The Hippo pathway is vital for organ growth control and tissue homeostasis, and its dysregulation has been linked to various human cancers. Upon activation MST1/2 phosphorylates LATS1/2 and MOB1 to support formation of an active MOB1/LATS complex, which phosphorylates YAP/TAZ, promoting its cytoplasmic retention and/or degradation. Thus, the Hippo core pathway can act through distinct kinases, with MOB1 acting as a fundamental signal adaptor that can interact with the Hippo core kinases MST1/2, LATS1/2, and NDR1/216, 19–22. Biochemical evidence suggests that MOB1 can associate with the highly conserved N-terminal regulatory domain (NTR) of NDR/LATS kinases to promote their activities.

To delineate the interaction of MOB1 with NDR2 on the atomic level, we determined the crystal structure of the MOB1/NDR2 complex at 2.1 Å using purified MOB1 (residues 33–216) and the NTR of NDR2 (residues 25–88). The structure of MOB1 adopts a globular shape consisting of nine α-helices (α1–α9) and two β-strands, as reported for unbound human MOB119, 32, frog MOB133, and yeast Mob1p34. The central intermolecular interactions between MOB1 and NDR2 are hydrogen bonds and van der Waals interactions, with the two antiparallel α-helices of NDR2 representing two interaction interfaces. In the α1 helix Lys25, Leu28, Tyr32, Leu35, and Ile36 of NDR2 interact with Leu36, Gly39, Leu41, Ala44, Gln67, Met70, Leu71, Leu173, Gln174, and His185 of MOB1. In the α2 helix Arg42, Leu78, Arg79, and Arg82 of NDR2 interact with Glu51, Glu55, Trp56, Val59, Phe132, Pro133, Lys135, and Val138 of MOB1. MOB1(Q67A) and MOB1(H185A) mutants did not interact with NDR2, illustrating that the observed MOB1/NDR2 interaction is specific. The overall crystal structure of MOB1 bound to NDR2 is very similar to the previously reported structures of MOB1/LATS119, 20. Most significantly, we discovered that His646 of LATS1 bonds with Asp63 of MOB1 supported by a cluster of surrounding residues involving Phe642, Met643, Gln645, Val647, and Val65019, while Phe31 of NDR2 does not interact with Asp63 of MOB1. Consequently, our structural comparison suggests that Asp63 of MOB1 specifically bonds with LATS kinases through His646, which is conserved in human LATS1/2 and fly Wts, but replaced by a bulky Phe/Tyr residue in human NDR1/2 and fly Trc. MOB1/NDR2 complex formation is dramatically increased by prior MST1/2 phosphorylation of MOB1, while the MOB1/LATS1 interaction appears to be fully dependent on MST1/2 phosphorylation of MOB1.

>AAHHSSGHMEATLGSGNLRQAVMLPEGEDLNEWIAVNTVDFFNQINMLYGTITEFCTEASCPVMSAGPRYEYHWADGTNIKKPIKCSAPKYIDYLMTWVQDQLDDETLFPSKIGVPFPKNFMSVAKTILKRLFRVYAHIYHQHFDSVMQLQEEAHLNTSFKHFIFFVQEFNLIDRRELAPLQELIEKLGSKDR[2x];>[2x]SSGHMKLTLENFYSNLILQHEERETRQKKLEVAMEEEGLADEEKKLRRSQHARKETEFLRLKRTRLGL>[3x]A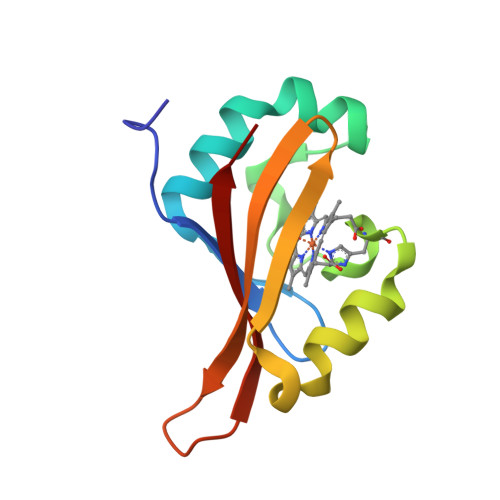VEGMTTNLMMADKEGIIQYLNPALLQLLTHREPELAQAFPGFKAAELVGKNIDIFHKNPAHQRSIISNPERLPFTSMIKVGSLEFNLTCIAMRDTKGEYIGPALQLVDIT> AVINHDAVPVWPQPEPADATQALAVRFKPQLDVVNGCQPYPAVDPQGNTSGGLKPSGSQAAACRDMSKAQVYSRSGTYNGYYAIMYSWYMPKDSPSTGIGHRHDWENVVVWLDNAASANIVALSA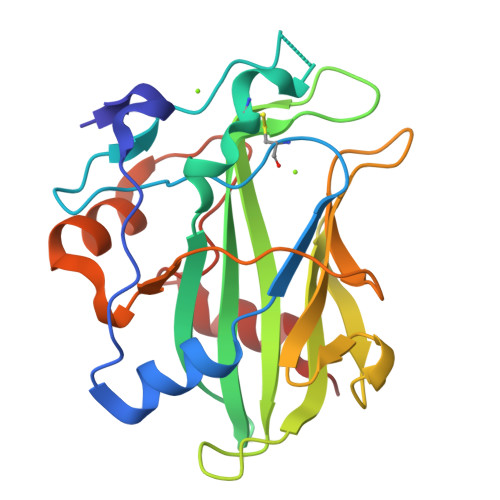SAHSGYKKSFPADKSYLDGITAKISYKSTWPLDHELGFTTSAGKQQPLIQWEQMTQAARDALESTDFGNANVPFKSNFQDKLVKAFFQ Hemolysin co-regulated protein 1 (Hcp1) is a component of the cluster 1 Type VI secretion system (T6SS1) that plays a key role during the intracellular lifecycle of Burkholderia pseudomallei. Hemolysin co-regulated protein 1 (Hcp1), encoded by bpss1498 (BPS_RS26895), is a component of T6SS1 and forms the secretion tube of this system that is necessary for the transport of effectors from the bacterial cytoplasm into host cells. One critical virulence factor expressed by B. pseudomallei is the cluster 1 Type VI secretion system (T6SS1) that has been shown to influence the intracellular behavior of this pathogen and be required for multinucleated giant cell (MNGC) formation. Hcp1 is recognized as a promising target antigen for developing melioidosis diagnostics and vaccines.

While the gene encoding Hcp1 is retained across B. pseudomallei strains, variants of hcp1 have recently been identified. The prevalence of hcp1 variants was assessed in 1,283 primary clinical B. pseudomallei isolates from 9 hospitals in Northeast Thailand, and in addition to wild-type Hcp1 (Hcp1wt), two variants designated variant A (Hcp1variant A) and variant B (Hcp1variant B) were identified. Sequence analysis of 1,283 primary clinical isolates of B. pseudomallei demonstrated the presence of 8 hcp1 alleles encoding three types of Hcp1 proteins, including Hcp1wt (98.05%), Hcp1variant A (1.87%) and Hcp1variant B (0.08%). Since Hcp1 is known to play a role in cell-to-cell spread in cell culture, the efficiency of multinucleated giant cell (MNGC) formation was determined using B. pseudomallei strains expressing the three different Hcp1 types. For control purposes, B. pseudomallei K96243 containing hcp1wt, hcp1variant A or hcp1variant B were constructed for use in these assays. Interestingly, when Hcp1variant A was expressed in B. pseudomallei K96243, this strain retained the ability to stimulate MNGC formation in A549 cells. In contrast, however, similar experiments with the Hcp1variant B demonstrated a decreased ability of B. pseudomallei to stimulate MNGC formation. Collectively, these results show that B. pseudomallei strains expressing variants of Hcp1 elicit variable antibody responses in melioidosis patients and differ in their ability to promote MNGC formation in cell culture.

>[2x]MAAHHHHHHLAGIYLKVKGKTTGEIKGSVVQEGHDGKIHILAFKNDYDMPARLQEGLTPAAAARGTITLTKEMDRSSPQFLQALGKREMMEEFEITIYSPKADKETGGDLTELLFTYKFEKVLITHMDQYSPTPHKDDSNGIKEGLLGYIEEIKFTYSGYSLEHAESGIAGAANWKNG> MGNEVAGVEDISVEIKPSSKRNSDARRTSRNVCSNEERKRRKYFHMLYLVCLMVHGFIRNEWINSKRLSRKLSNLVPEKVFELLHPQKDEELPLRSTRKLLDGLKKCMELWQKHWKITKKYDNEGLYMRTWKEIEMSANNKRKFKTLKRSDFLRAVSKGHGDPDISVQGFVAMLRACNVNARLIMSCQPPDFTNMKIDTSLNGNNAYKDMVKYPIFWCEVWDKFSKKWITVDPVNLKTIEQVRLHSKLAPKGVACCERNMLRYVIAYDRKYGCRDVTRRYAQWMNSKVRKRRITKDDFGEKWFRKVITALHHRKRTKIDDYEDQYFFQRDESEGIPDSVQDLKNHPYYVLEQDIKQTQIVKPGCKECGYLKVHGKVGKVLKVYAKRDIADLKSARQWYMNGRILKTGSRCKKVIKRTVGRPKGEAEEEDERLYSFEDTELYIPPLASASGEITKNTFGNIEVFAPTMIPGNCCLVENPVAIKAARFLGVEFAPAVTSFKFERGSTVKPVLSGIVVAKWLREAIETAIDGIEFI;> GSGNASSGALGTTG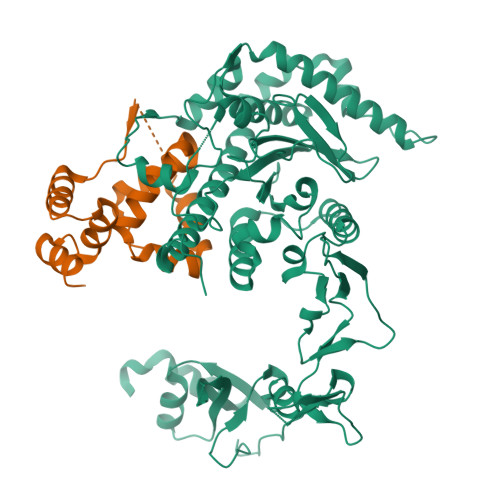GATDAAQGGPPGSIGLTVEDLLSLRQVVSGNPEALAPLLENISARYPQLREHIMANPEVFVSMLLEAVGDNMQDVMEGADDMVEGEDIEVTGEAAAAGLGQGEGEGSFQVDYTPEDDQAISRLCELGFERDLVIQVYFACDKNEEAAANILFSDHAD> MGHHHHHHKVTLPDLKWDFGALEPYISGQINELHYTKHHQTYVNGFNTAVDQFQELSDLLAKEPSPANARKMI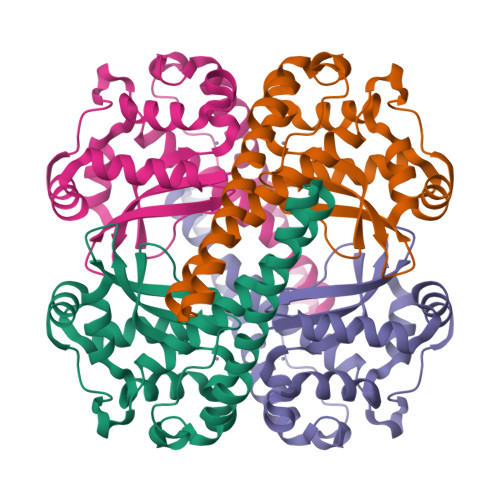AIQQNIKFHGGGFTNHCLFWENLAPESQGGGEPPTGALAKAIDEQFGSLDELIKLTNTKLAGVQGSGWAFIVKNLSNGGKLDVVQTYNQDTVTGPLVPLVAIDAWEHAYYLQYQNKKADYFKAIWNVVNWKEASRRFDAGKI>[3x]GSDEYDYLFKVVLIGDSGVGKSNLLSRFTRNEFNLESKSTIGVEFATRSIQVDGKTIKAQIWDTAG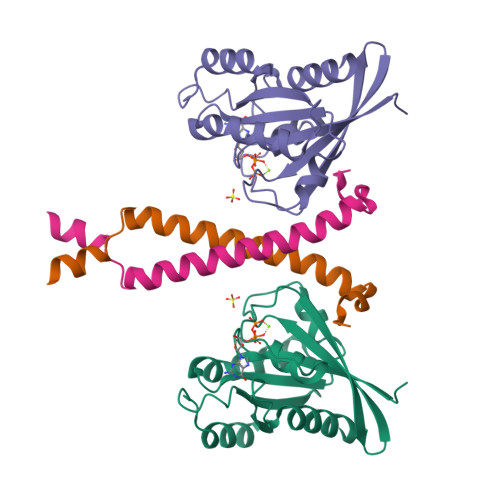LERYRAITSAYYRGAVGALLVYDIAKHLTYENVERWLKELRDHADSNIVIMLVGNKSDLRHLRAVPTDEARAFAEKNGLSFIETSALDSTNVEAAFQTILTEIYRI;>GSGAKSLFSTAFSESLAAEISSVSRDELMEAIQKQEEINFRLQDYIDRIIVAIMETNPSILEVK[3x]>EFPFALEVQTLPQTCDGPKAHTSFQISLSVSYI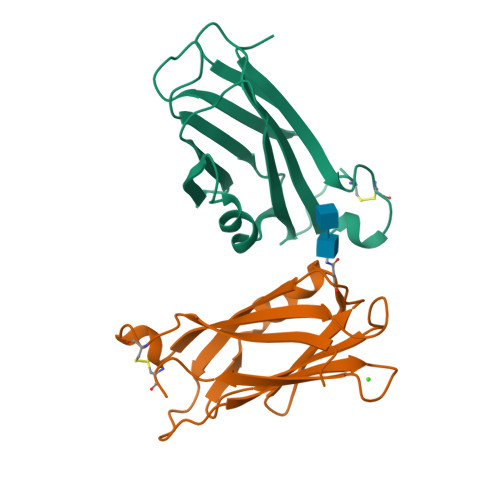GSRPASNMAIVDVKMVSGFIPLKPTVKMLERSNVSRTEVSNNHVLIYLDKVTNETLTLTFTVLQDIPVRDLKPAIVKVYDYYETDEFAVAEYSAPCS[2x]> GAMSTTSTTIQVIGAGLPRTGTNSMKKALEIIYSKPCYHMYEIIFKKQSDISIWQQLIDETHKTTSDKRKIYNGLNELLNGYIATTDLPSCSFYKELMTMYPNAKVLLTIRDKYDWLYSLRKVVLPKSTDPWKLKIEEGDQVLGIDSNFYKMTEDSLKFAFQKNHINLDDDEILLECYDEYNRLVQEIVPPERLLIHHLGDGWESLCQFLN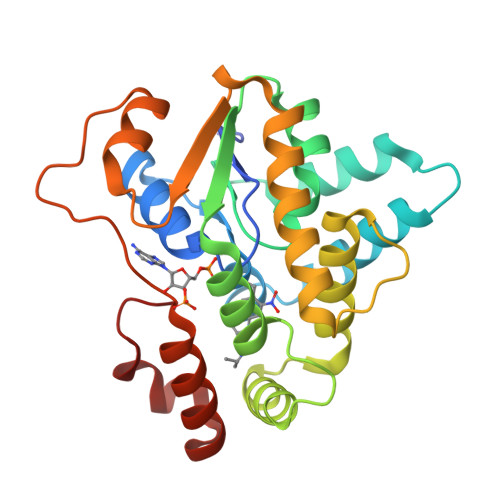VDIPNGISYPCANSHHQMTQLTEQLIKHKSLDDIIHMFPGLI>[4x]MTGLVQRCVIIQKDQHGFGFTVSGDRIVLV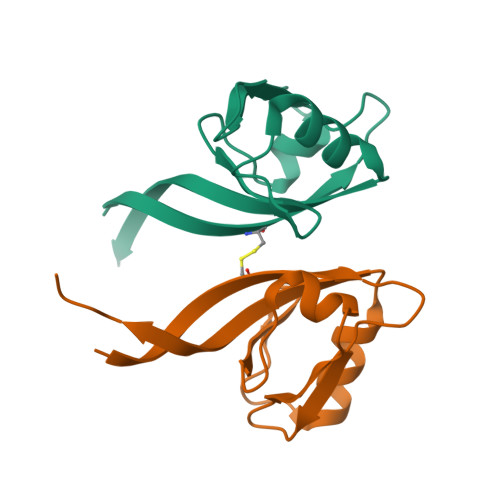QSVRPGGAAMKAGVKEGDRIIKVNGTMVTNSSHLEVVKLIKSGAYVALTLLGSSTSTTL Universally conserved across the three domains of life, enolase (EC 4.2.1.11) is an essential enzyme that catalyses the dehydration of 2-phospho-d-glycerate to phosphoenol­pyruvate in glycolysis and the reverse reaction in gluconeogenesis. In addition to playing a primary role in metabolism, enolases have evolved an impressive range of ‘moonlighting’ functions. Toxoplasma possesses two enolase isoforms that are differentially expressed in a stage-specific manner. Enolase 2 (TgENO2) has been shown to be specifically expressed in tachyzoites, whereas enolase 1 (TgENO1) is solely expressed in bradyzoites.

An apo TgENO1 crystal structure was determined in space group I4 to 2.75 Å resolution. The crystallographic asymmetric unit contained three nearly identical TgENO1 homodimers. The TgENO1 structure reveals that the two plant-like enolase insertions are located on surface loops. The larger pentapeptide insertion EWGYS forms a short β-strand (β5) between the α3 and α4 helices. The insertion produces a more positively charged surface potential at this N-terminal domain loop. The dipeptide insertion KQ, which is between β11 and β12, also increases the charged surface potential of loop L3 in the C-terminal domain, providing a possible site for binding to ligands that will negatively regulate the catalytic pocket. The interaction of the N-terminal domain of one subunit with the C-terminal domain of the other subunit forms the TgENO1 dimer interface that buries 1891.7 Å2 and contains 33 hydrogen bonds and 15 salt bridges. While key catalytic and ligand-binding residues (TgENO1/human ENO1: His165/159, Glu174/168, Glu217/211, Lys355/345 and Lys406/396) are conserved, TgENO1 exhibits three atypical residues (Glu164, Leu176 and Gln380) in the active-site pocket in comparison to TgENO2 and other enolases. Most notable in the bradyzoite TgENO1 is the presence of Glu164 at a position that is most commonly occupied by a serine in other enolases. However, a comparison of calculated surface electrostatic potentials indicates that the nuclear enolases (hENO1 and TgENO1) tend to have a higher degree of positive potential than the cytoplasmic enolases (hENO2, Streptococcus pneumoniae ENO1).

>[6x]MVVIKDIVAREILDSRGNPTIEVDVSTEGGVFRAAVPSGASTGIYEALELRDKDPKRYLGKGVLNAVEIVRQEIKPALLGKDPCDQKGIDMLMVEQLDGTKNEWGYSKSKLGANAILGVSIACCRAGAASKGLPLYKYIATLAGKTIDKMVMPVPFFNVINGGEHAGNGLALQEFLIAPVGAPNIREAIRYGSETYHHLKNVIKNKYGLDATNVGDEGGFAPNVATAEEALNLLVEAIKAAGYEGKIKIAFDAAASEFYKQDEKKYDLDYKCKTKNASKHLTGEKLKEVYEGWLKKYPIISVEDPFDQDDFASFSAFTKDVGEKTQVIGDDILVTNILRIEKALKDKACNCLLLKVNQIGSVTEAIEACLLAQKSGWGVQVSHRSGETEDSFIADLVVGLRCGQIKSGSPCRSERLCKYNQLMRIEESLGADCVYAGESFRHPKRSHHHHHH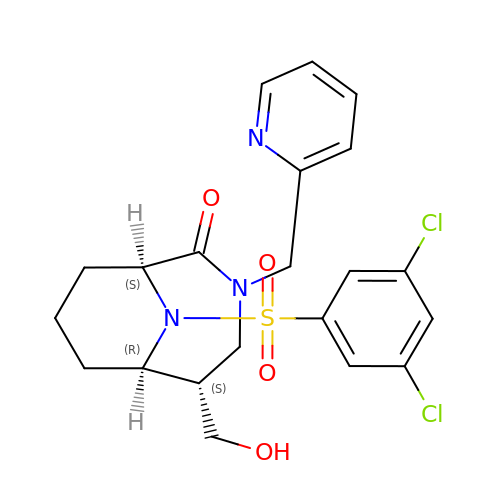(1~{S},5~{S},6~{R})-10-[3,5-bis(chloranyl)phenyl]sulfonyl-5-(hydroxymethyl)-3-(pyridin-2-ylmethyl)-3,10-diazabicyclo[4.3.1]decan-2-one | C21 H23 Cl2 N3 O4 S | SLQCBVGDPHQIBY-XMCHAPAWSA-N> SDRVRSITLGNSTITTQESANVVVGYGRWPEYLRDDEATAEDQPTQPDVATCRFYTLESVTWEKDSPGWWWKFPDALKDMGLFGQNMYYHYLGRAGYTIHVQCNASKFHQGCLLVVCVPEAEMGCSTVDGTVNEHGLSEGETAKKFSATGTNGTNTVQSIVTNAGMGVGVGNLTIFPHQW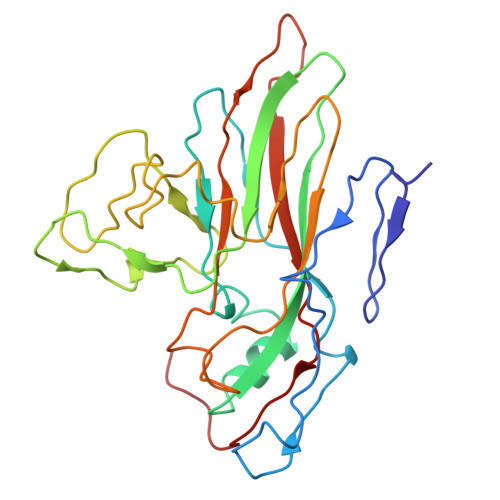INLRTNNCATIVMPYINNVPMDNMFRHHNFTLMIIPFVPLNYSSDFSTYVPITVTVAPMCAEYNGLRLSTAL> VTKPTIAAVGGYAMNNGTGTTLYTKAADTRRSTGSTTHIMTA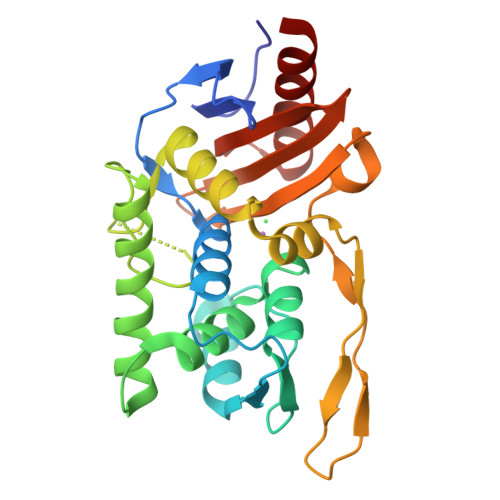KVVLAQSNLNLDAKVTIQKAYSDYVVANNASQAHLIVGDKVTVRQLLYGLMLPSGCDAAYALADKYGSGSTRAARVKSFIGKMNTAATNLGLHNTHFDSFDGIGNGANYSTPRDLTKIASSAMKNSTFRTVVKTKAYTAKTVTKTGSIRTMDTWKNTNGLLSSYSGAIGVKTGSGPEAKYCLVFAATRGGKTVIGTVLASTSIPARESDATKIMNYGFAL> FACKTANGTAIPIGGGSANVYVNLAPVVNVGQNLVVDLSTQIFCHNDYPETITDYVTLQRGSAYGGVLSNFSGTVKYSGSSYPFPTTSETPRVVYNSRTDKPWPVALYLTPVSSAGGVAIKAGSLIAVLILRQTNNYNSDD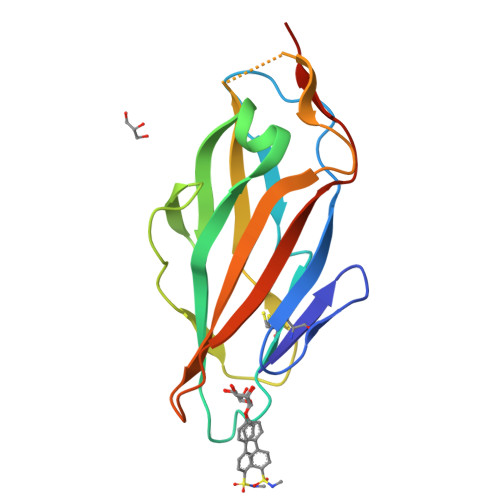FQFVWNIYANNDVVVPTGLVPR> MGWDLTVKMLAGNEFQVSLSSSMSVSELKAQITQKIGVHAFQQRLAVHPSGVALQDRVPLASQGLGPGSTVLLVVDKSDEPLSILVRNNKGRSSTYEVRLTQTVAHLKQQVSGLEGVQDDLFWLTFEGKPLEDQLPLGEYGLKPLSTVFMNLRLRGGGR;> MADNMTTTQIEVGPGATNATINFEAGILECYERFSWQRALDYPGQDRLHRLKRKLESRI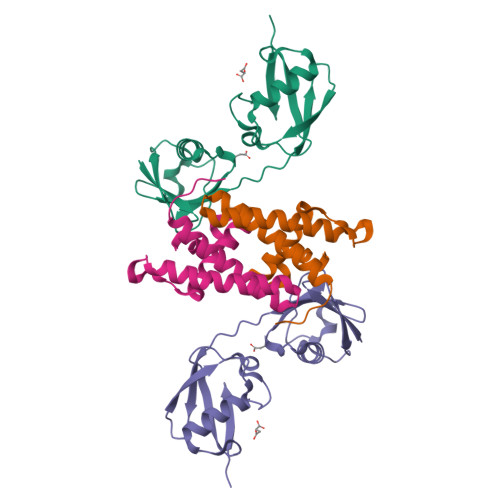KTHNKSEPENKRMSLEERKAIGVKMMKVLLFMDPSAGIEGFEPYHHHHHH>APVTSPAWADDPPATVYRYDSRPPEDVFQNGFTAWGNNDNVLEHLTGRSCQVGSSNSAFVSTSSSRRYTEVYLEHRMQEAVEAERAGRGTGHFIGYIYEVRADNNFYGAASSYFEYVDTYGDNAGRILAGALATYQSEYLAHRRIPPENIRRVTRVYHNGITGETTTTEYSNARYVSQQTRANPNPYTSRRSVASIVGTLVRMAPVVGACMARQAESSEAMAAWSERAGEAMVLVYYESIAYSF[2x];> GIVIPPQEQITQHGSPYGRCANKTRALTVAELRGSGDLQEYLRHVTRGWSIFALYDGTYLGGEYGGVIKDGTPGGAFDLKTTFCIMTTRNTGQPATDHYYSNVTATRLLSSTNSRLCAVFVRSGQPVIGACTSPYDGKYWSMYSRLRKMLYLIYVAGISVRVHVSKEEQYYDYEDATFETYALTGISICNPGSSLC;>GIVIPPKALFTQQGGAYGRCPNGTRALTVAELRGNAELQT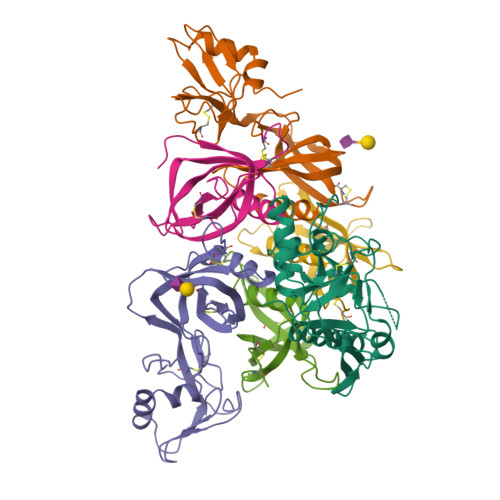YLRQITPGWSIYGLYDGTYLGQAYGGIIKDAPPGAGFIYRETFCITTIYKTGQPAADHYYSKVTATRLLASTNSRLCAVFVRDGQSVIGACASPYEGRYRDMYDALRRLLYMIYMSGLAVRVHVSKEEQYYDYEDATFQTYALTGISLCNPAASIC[2x];>DVPYVLVKTNMVVTSVAMKPYEVTPTRMLVCGIAAKLGAAASSPDAHVPFCFGKDLKRPGSSPMEVMLRAVFMQQRPLRMFLGPKQLTFEGKPALELIRMVECSGKQDCP[4x];>LPTHLYKNFTVQELALKLKGKNQEFCLTAFMSGRSLVRACLSDAGHEHDTWFDTMLGFAISAYALKSRIALTVEDSPYPGTPGDLLELQICPLNGYCE[2x];> TPGIVIPPQEQITQHGSPYGRCANKTRALTVAELRGSGDLQEYLRHVTRGWSIFALYDGTYLGGEYGGVIKDGTPGGAFDLKTTFCIMTTRNTGQPATDHYYSNVTATRLLSSTNSRLCAVFVRSGQPVIGACTSPYDGKYWSMYSRLRKMLYLIYVAGISVRVHVSKEEQYYDYEDATFETYALTGISICNPGSSLC>[3x]MSTPARRRLMRDFKRMKEDAPPGVSASPLPDNVMVWNAMIIGPADTPYEDGTFR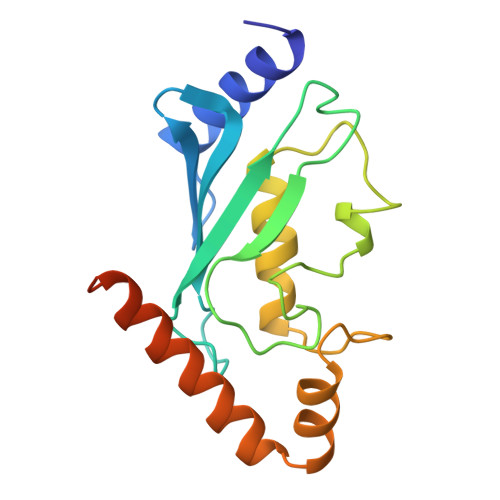LLLEFDEEYPNKPPHVKFLSEMFHPNVYANGEICLDILQNRWTPTYDVASILTSIQSLFNDPNPASPANVEAATLFKDHKSQYVKRVKETVEKSWEDDMDDDDDDDDDDDDDEAD>IFAEDV[4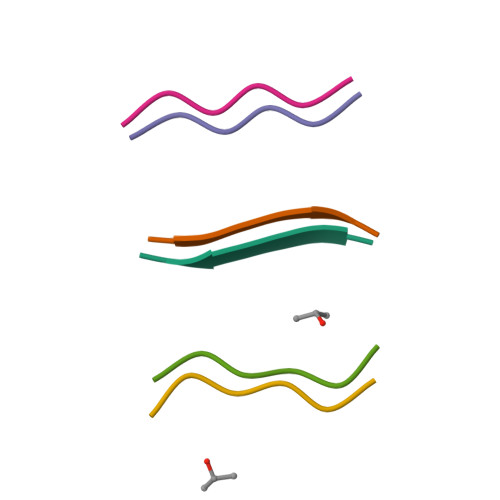x]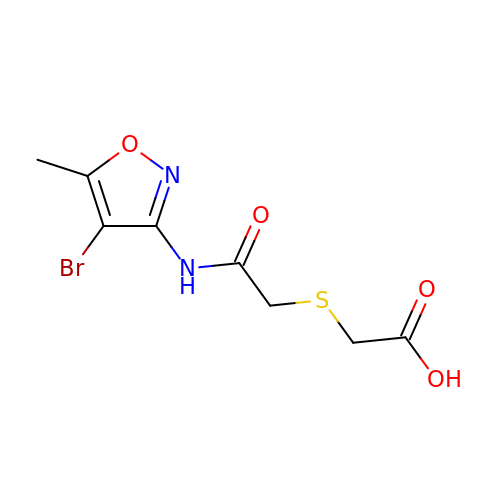({2-[(4-bromo-5-methyl-1,2-oxazol-3-yl)amino]-2-oxoethyl}sulfanyl)acetic acid | C8 H9 Br N2 O4 S | CMJFFJICEDWDAG-UHFFFAOYSA-N> DNLRHFVQDYAVR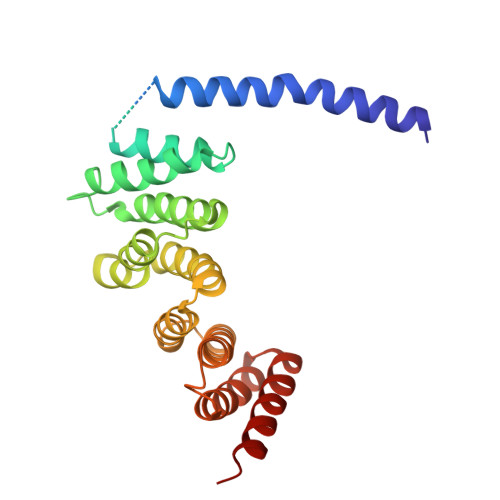ALIPYIEHLVAILAEGVTNKKGVSKSLLSATKRWFVTSKPGAGANNQNAVIYTNESAELQTRKLGDLYFMFGHYNLAFQSYHQAKRDFNADSAWQYYAGALEMAALSAFMLGTAQRKTYDYMEDAIVCYLTVCKLQQFATRATLLSMECLKTARLYSEVAKQLIRMTNEESDLRSALLLEQAAYCFLVTQPPMHRKYAFHIVLAGNRYSRAGQRKHAYRCYRQAYQVFQKREW(2R,3S)-1,4-DIMERCAPTOBUTANE-2,3-DIOL | C4 H10 O2 S2 | 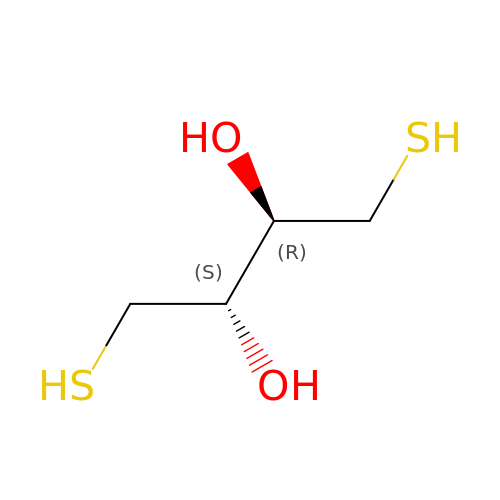VHJLVAABSRFDPM-ZXZARUISSA-N>[2x]GGSWEIDPKDLTFLKELGTGQFGVVKYGKWRGQYDVAIKMIKEGSMSEDEFIEEAKVMMNLSHEKLVQLYGVCT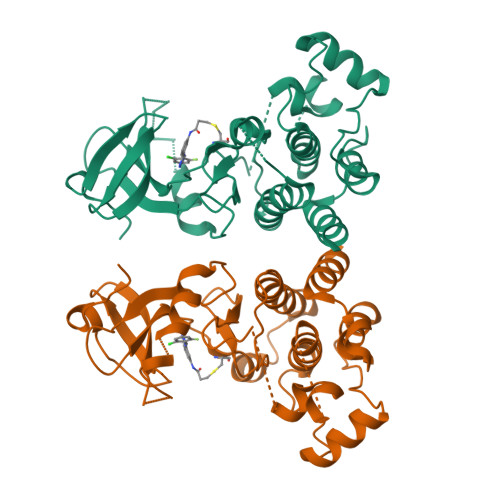KQRPIFIITEYMANGCLLNYLREMRHRFQTQQLLEMCKDVCEAMEYLESKQFLHRDLAARNCLVNDQGVVKVSDFGLSRYVLDDEYTSSVGSKFPVRWSPPEVLMYSKFSSKSDIWAFGVLMWEIYSLGKMPYERFTNSETAEHIAQGLRLYRPHLASEKVYTIMYSCWHEKADERPTFKILLSNILDVMD> GAEQQADTVTENSDSEVFVDDSDRFTAFEEEL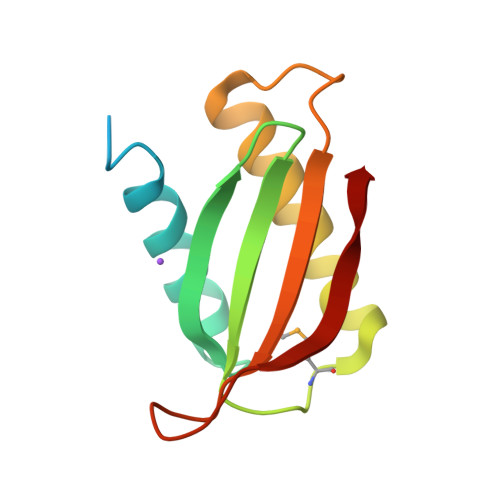LARYADKGIRSVDVAAYAKGIDIVFVAADRKMTRAEFSAIASRSIRELKERFGFDKDVPIGAVLDYKKDAATDTRTRFVLKLR> MKLKILDKDNATLNVFHRNKEHKTIDNVPTANLVDWYPLSNAYEYKLSRNGEYLELKRLRSTLPSSYGLDDNNQDIIRDNNHRCKIGYWYNPAVRKDNLKIIEKAKQYGLPIITEEYDANTVEQGFRDIGVIFQSLKTIVVTRYLEGKTEEELRIFNMKSEES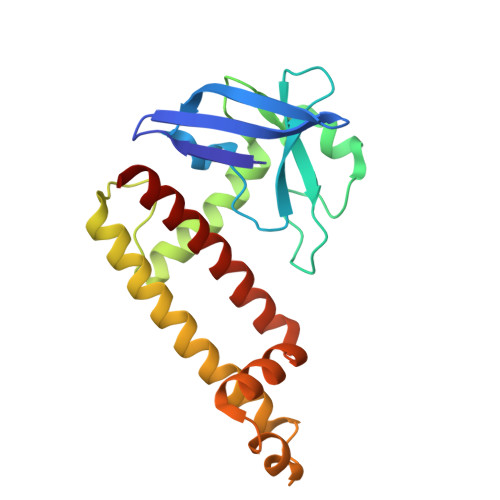QLNEALKESDFSVDLTYSDLGQIYNMLLLMKKISK> SKNRISWVGDAVKTDGKKSYYKKVCIDSETLEVGDCVSVIPDDSSKPLYLARVTALWEDSSNGQMF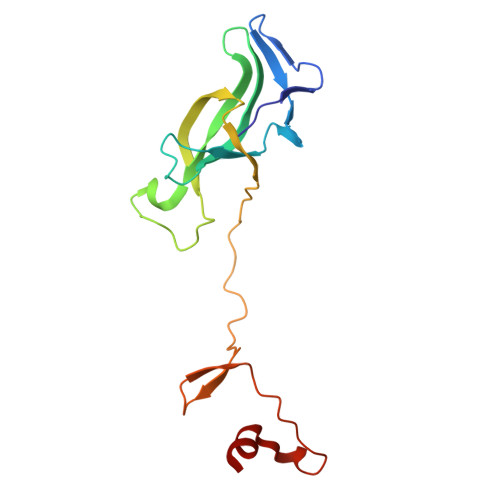HAHWFCAGTDTVLGATSDPLELFLVDECEDMQLSYIHSKVQVIYKAPSGAGSATYFYQLWYDQDYARFESPPKTQPTEDNKYKFCASCARLA>[2x]EAEAAGLNTAAKAKGLKYFGSATDNPELTDSAYVAQLSNTDDFGQITPGNSMKWDATEPSQNSFSFANGDAVVNLANKNGQLMRCHTLVWHSQLPNWVSSGSWTNATLLAAMKNHITNVVTHYKGKCYAWDVVNEALNEDGTFRNSVFYQIIGPAYIPIAFATAAAADPDVKLYYNDYNIEYSGAKATAAQNIVKMIKAYGAKID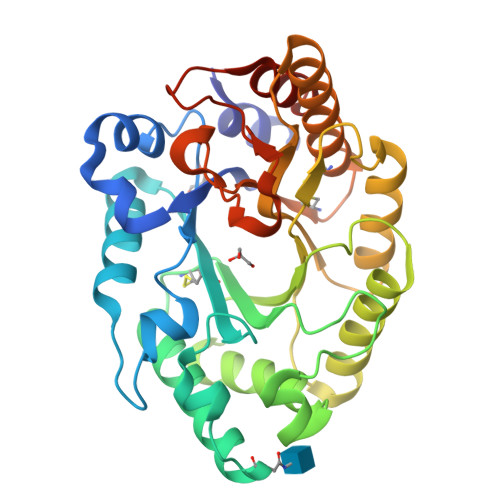GVGLQAHFIVGSTPSQSDLTTVLKGYTALGVEVAYTELDIKMQLPSTAAKLAQQSTDFQGVAAACVSTTGCVGVTIWDWTDKYSWVPSVFQGYGAPLPWDENYVKKPAYDGLMAGLGASGSGTT(1S,2S,3R,6R)-6-[(4-phenoxybenzyl)amino]cyclohex-4-ene-1,2,3-triol 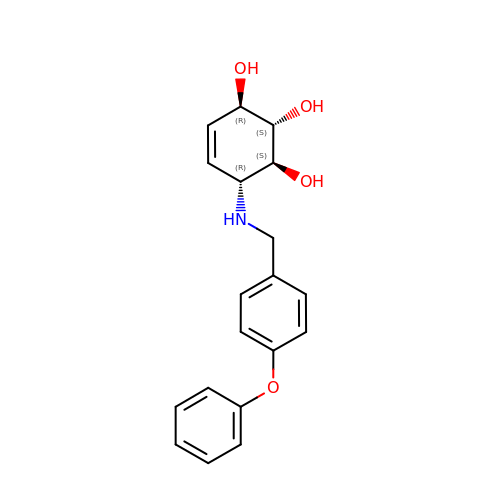| C19 H21 N O4 | YNNCSTZOAWTUPJ-YRXWBPOGSA-N> MRVLGIETSCDATGIAIYDDEKGLLANQLYSQVKLHADYGGVVPELASRDHVRKTVPLIQAALKESGLTAKDIDAVAYTAGPGLVGALLVGATVGRSLAFAWDVPAIPVHHMEGHLLAPMLEDNPPEFPFVALLVSGGHTQLISVTGIGQYELLGESIDDAAG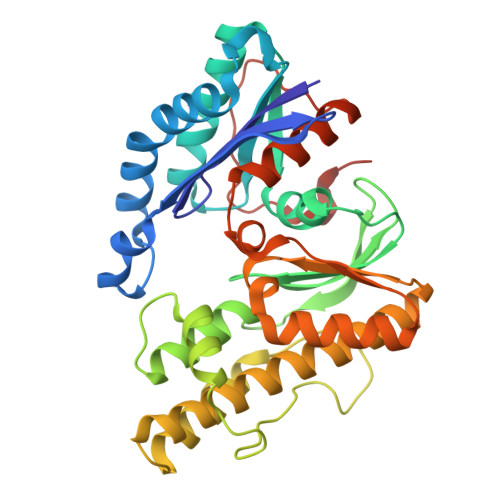EAFDKTAKLLGLDYPGGPLLSKMAAQGTAGRFVFPRPMTDRPGLDFSFSGLKTFAANTIRDNGTDDQTRADIARAFEDAVVDTLMIKCKRALDQTGFKRLVMAGGVSANRTLRAKLAEMMKKRRGEVFYARPEFCTDNGAMIAYAGMVRFKAGATADLGVSVRPRWPLAELPAAHHHHHH TBEV belongs to the family Flaviviridae of positive-sense, single-stranded RNA viruses. Here, we report the structures of the native TBEV virion and its complex with the Fab fragments of the neutralizing antibody 19/1786. In contrast to the principles suggested by Caspar and Klug and unlike most isometric viruses, the three E-protein subunits within one icosahedral asymmetric unit form unique interactions with the surrounding glycoproteins. Both E-proteins and M-proteins are anchored in the virion membrane, each by two trans-membrane helices. Two M-proteins and two E-proteins form a heterotetramer in which each M-protein interacts with both E-proteins.

Nevertheless, the structure of the mature TBEV particle was determined to a resolution of 3.9 Å. The quality of the map was sufficient to enable the building of the protein components of the TBEV envelope, which contains three E-proteins and three M-proteins in each icosahedral asymmetric unit. The surface of the TBEV virion is covered with small protrusions formed by glycans attached to the E-protein subunits. Three of these heterotetramers constitute the so-called herringbone pattern characteristic of the envelopes of flaviviruses. The cryo-EM reconstruction contains densities corresponding to N-acetyl-D-glucosamine in all three E-protein subunits of the asymmetric unit. Whereas in the crystal structure the domains I, II, and III are arranged in a line, in the virion the tip of domain II is bent 15 Å toward the virus membrane. The bending of the ectodomain in the virion is necessary to keep the fusion loop buried in the hydrophobic pocket of the other E-protein from the same dimer, so that the loop is prevented from untimely induction of membrane fusion. The N-terminal loop of the M-protein interacts with domain II of the E-protein and presumably prevents the reorganization of E-protein dimers into fusogenic trimers. TBEV homologs His7 and His216 are located 5.9 Å away from each other, and are therefore likely to have the same function in sensing low pH. Repulsion between these amino acids is likely to trigger the release of ectodomains of E-proteins from the virus envelope, enabling the formation of fusion trimers.

>[3x]SRCTHLENRDFVTGTQGTTRVTLVLELGGCVTITAEGKPSMDVWLDAIYQENPAQTREYCLHAKLSDTKVAARCPTMGPATLAEEHQGGTVCKRDQSDRGWGNHCGLFGKGSIVACVKAACEAKKKATGHVYDANKIVYTVKVEPHTGDYVAANETHSGRKTASFTVSSEKTILTMGEYGDVSLLCRVASGVDLAQTVILELDKTVEHLPTAWQVHRDWFNDLALPWKHEGARNWNNAERLVEFGAPHAVKMDVYNLGDQTGVLLKALAGVPVAHIEGTKYHLKSGHVTCEVGLEKLKMKGLTYTMCDKTKFTWKRAPTDSGHDTVVMEVTFSGTKPCRIPVRAVAHGSPDVNVAMLITPNPTIENNGGGFIEMQLPPGDNIIYVGELSYQWFQKGSSIGRVFQKTKKGIERLTVIGEHAWDFGSAGGFLSSIGKALHTVLGGAFNSIFGGVGFLPKLLLGVALAWLGLNMRNPTMSMSFLLAGVLVLAMTLGVGA;>[3x]SVLIPSHAQGELTGRGHKWLEGDSLRTHLTRVEGWVWKNRLLALAMVTVVWLTLESVVTRVAVLVVLLCLAPVYA1-benzothiophene-7-carboxylic 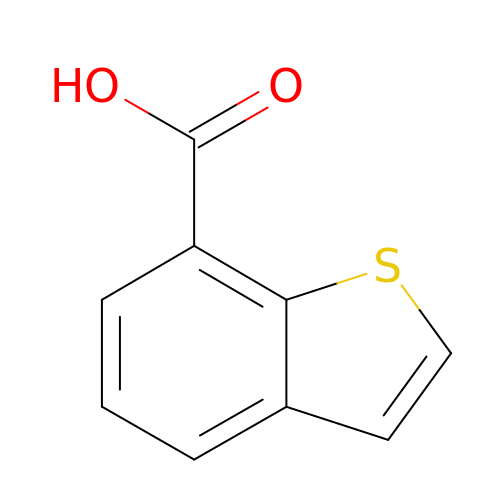acid | C9 H6 O2 S | LJPSRTWIAXVPIS-UHFFFAOYSA-N>MGHHHHHHEFEKSIPICTLKNFPNAIEHTLQWARDEFEGLFKQPAENVNQYLTDSKFVERTLRLAGTQPLEVLEAVQ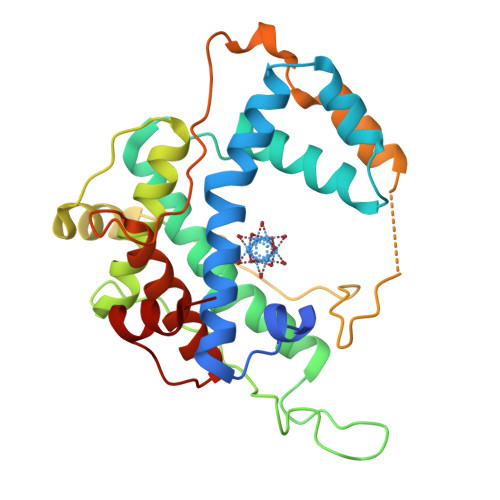RSLVLQRPQTWGDCVTWACHHWHTQYCNNIRQLLHNFPPDQLTSSGAPFWSGPKRCPHPLTFDVNNTLHLDYVMAAANLFAQTYGLTGSQDRAAVASLLQSVQVPEFTPKSGVKIHVSDQELQSANASVDDSRLEELKATLPSPDKLPGFKMYPIDFEKDDDSNFHMDFIVAASNLRAENYDISPADRHKSKLIAGKII[3x]> ADVTITVNGKVVA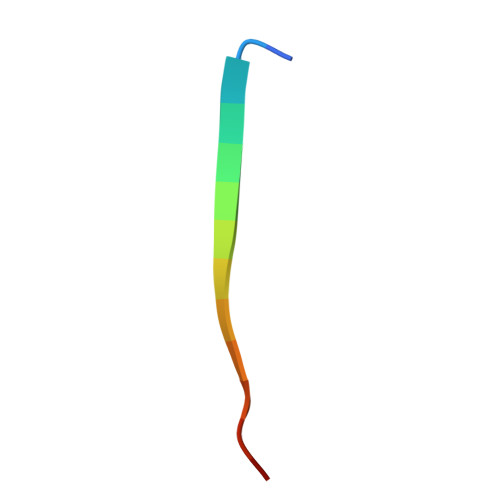K> MGSDKIHHHHHHENLYFQGAVDLDREGRDPAYVESIVKRSQKIVDKLELTDTVAAREVTTIIANRYFKLNDIYETRDAKVKLAKETLTGDAKQEAVKAAEAEKDAALYRTH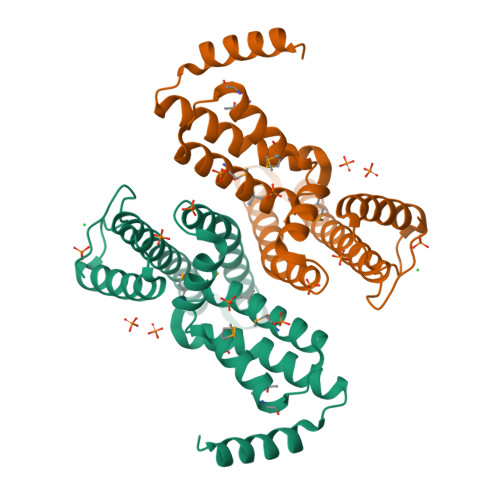FAFPADLSLYLDAKQIDAVKDGMTYGVVMVTYKATVDMIPTLKEEEKAQIMAWLVEAREFAMDAENSNKKHAAFGKYKGRINNYLSKRGYDLVKERKAWYERIKARGGKI> SEEMIDHRLTDREWAEEWKHLDHLLNCIMDMVEKTRRSLTVL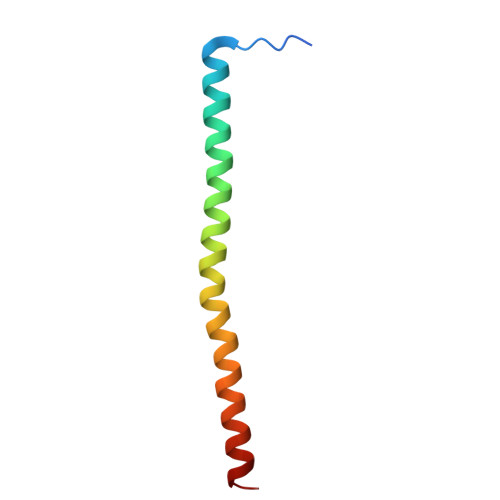RRCQEADREELNYWIRRYSDAE> GVAAPQNYLAVIKVVGIGGGGVNAVNRMIEEGLKGVEFIAINTDAQALLMSDADVKLDVGRELTRGLGAGANPDVGRKAAEDHREEIEEVLKGADMVFVTAGEGGG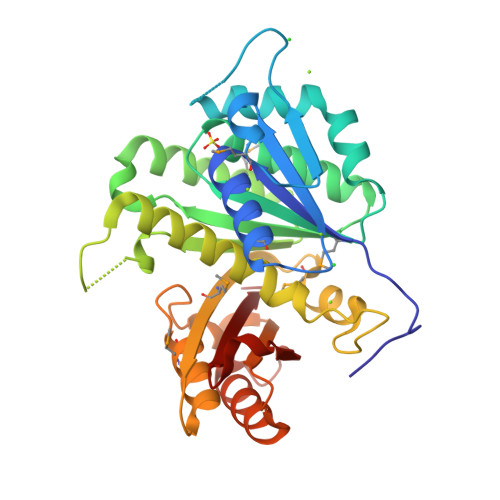TGTGGAPVVANIARSLGALTIGVVTRPFSFEGKRRATQAEAGIAMLREEVDTLIVIPNDRLLSISDRQVSVLDAFKAADQVLLSGVQGITDLITTPGLINLDFADVKSVMSGAGSALMGIGSARGDDRAVAAAEMAISSPLLEASIDGAHGVLLSIQGGSDLGLFEINEAAQLVANSAAAEANIIFGAVIDDALGDEVRVTVIAAGFD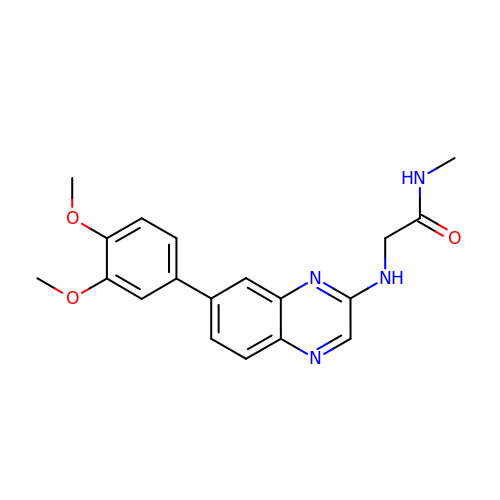N~2~-[7-(3,4-dimethoxyphenyl)quinoxalin-2-yl]-N-methylglycinamide | C19 H20 N4 O3 | LYPCULYCGFOIDA-UHFFFAOYSA-N4-(4-{[(2-chloro-6-fluorophenyl)carbamoyl]amino}-1H-pyrazol-1-yl)-N-(oxetan-3-yl)thiophene-2-carboxamide 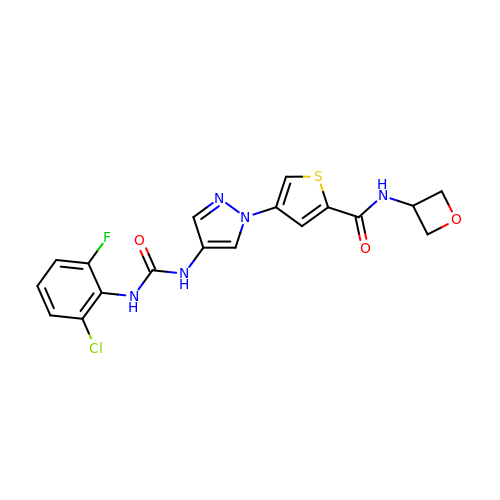| C18 H15 Cl F N5 O3 S | ANCCTLHKRLRSAF-UHFFFAOYSA-N>[3x]TARVKRGMAEMLKGGVIMDVVTPEQARIAEGAGAVAVMALERVPADIRAQGGVSRMSDPDMIEGIIAAVTIPVMAKVRIGHFVEAQILQTLGVDYIDESEVLTPADYAHHIDKWNFTVPFVCGATNLGEALRRI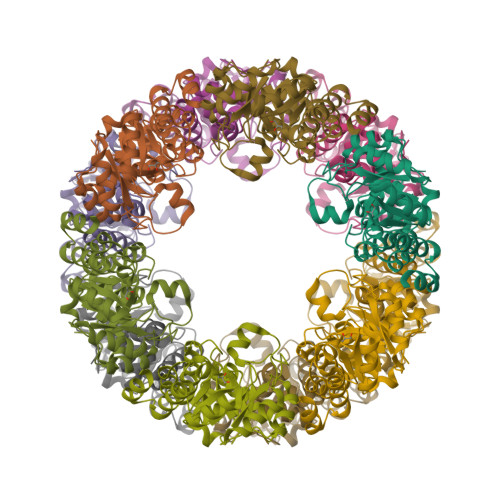SEGAAMIRSKGEAGTGDVSNATTHMRAIGGEIRRLTSMSEDELFVAAKELQAPYELVAEVARAGKLPVTLFTAGGIATPADAAMMMQLGAEGVFVGSGIFKSGAPEHRAAAIVKATTFFDDPDVLAKVSR>[4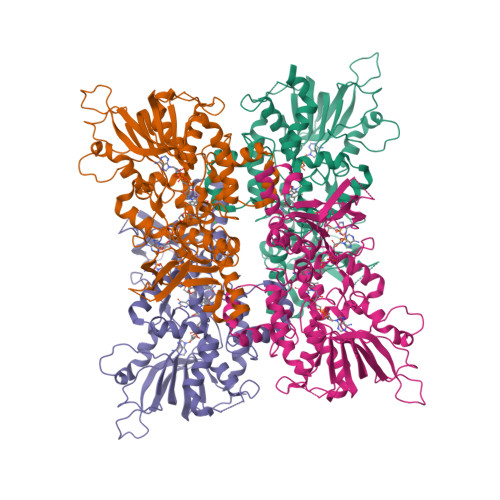x]MESVERKSESSYLGMRNMQPEQRLSLDPPRLRSTPQDELHDLLCVGFGPASLAIAIALHDALDPRLNKSASNIHAQPKICFLERQKQFAWHSGMLVPGSKMQISFIKDLATLRDPRSSFTFLNYLHQKGRLIHFTNLSTFLPARLEFEDYMRWCAQQFSDVVAYGEEVVEVIPGKSDPSSSVVDFFTVRSRNVETGEISARRTRKVVIAIGGTAKMPSGLPQDPRIIHSSKYCTTLPALLKDKSKPYNIAVLGSGQSAAEIFHDLQKRYPNSRTTLIMRDSAMRPSDDSPFVNEIFNPERVDKFYSQSAAERQRSLLADKATNYSVVRLELIEEIYNDMYLQRVKNPDETQWQHRILPERKITRVEHHGPQSRMRIHLKSSKPESEGAANDVKETLEVDALMVATGYNRNAHERLLSKVQHLRPTGQDQWKPHRDYRVEMDPSKVSSEAGIWLQGCNERTHGLSDSLLSVLAVRGGEMVQSIFGEQLERAAVQGHQLRAML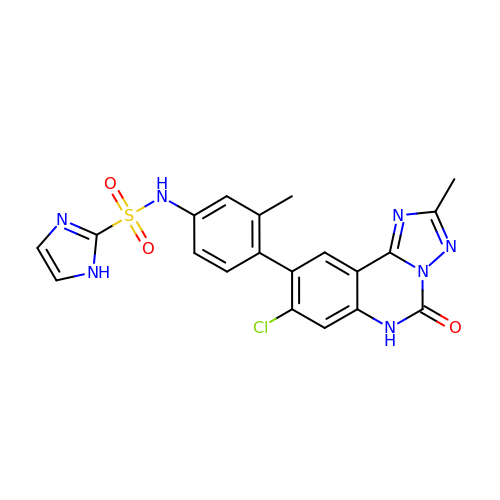N-{4-[(4S,10aP)-8-chloro-2-methyl-5-oxo-5,6-dihydro[1,2,4]triazolo[1,5-c]quinazolin-9-yl]-3-methylphenyl}-1H-imidazole-2-sulfonamide | C20 H16 Cl N7 O3 S | MJDFVGVHKKUOFT-UHFFFAOYSA-N>[2x]GSSGSSGIGEGMLADFVSQTSPMIPSIVVHCVNEIEQRGLTETGLYRIAGCDRTVKELKE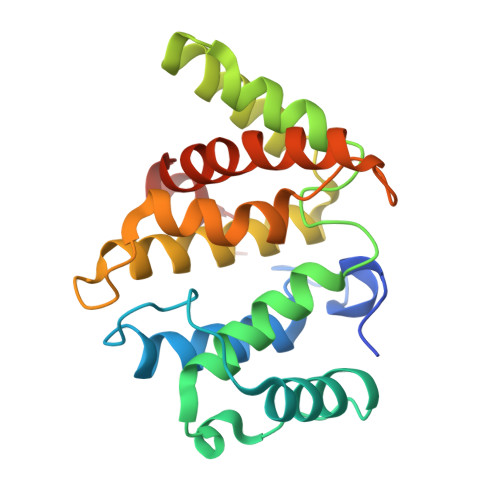KFLRVKTVPLLSKVDDIHAICSLLKDFLRNLKEPLLTFRLNRAFMEAAEITDEDNSIAAMYQAVGELPQANRDTLAFLMIHLQRVAQSPHTKMDVANLAKVFGPTIVAHAVPNPDPVTMSQDIKRQPKVVERLLSLPLEYWSQFMMVE~{N}-[(3~{S})-1-(4-chlorophenyl)-2,5-bis(oxidanylidene)pyrrolidin-3-yl]-~{N}-oxidanyl-hexanamide | C16 H19 Cl N2 O4 | 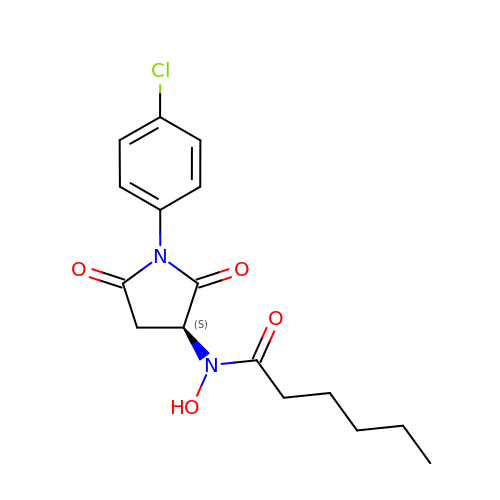ZAMVBYSBDZJLIX-ZDUSSCGKSA-N(2S)-2-aminoheptanedioic 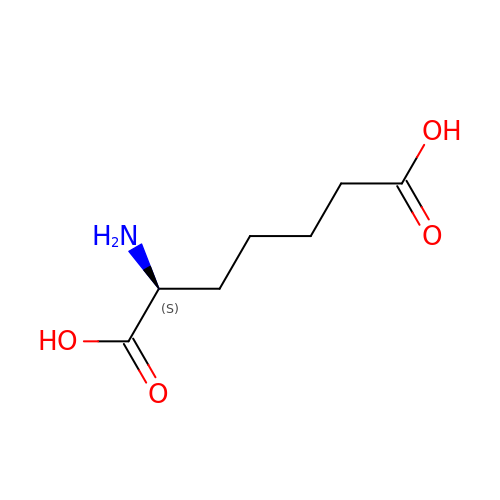acid | C7 H13 N O4 | JUQLUIFNNFIIKC-YFKPBYRVSA-N>PAAELEARQFDPDSFKNKWLELHNNERT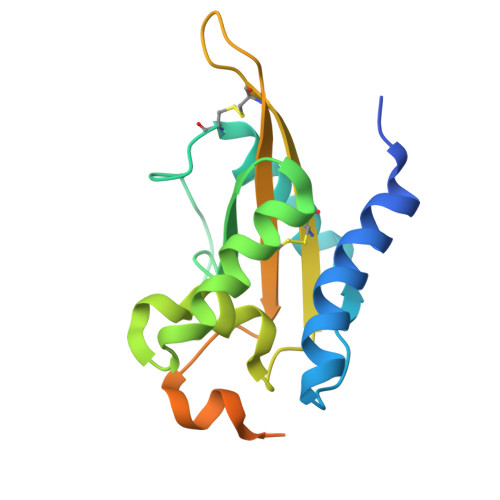TRQLDSLEWDGDLAWKAQQVATQCNVDNPQLWGDNGASFNIGRYTKEQAFAEWTATSGSFPDDRSIPWQRIVANSAQKVGCGEATCVLEGDMAYTVNVCYYDPPLSDYYTNAGDNVRVPSLALLNLDLTTPFCNLPVNGSNDLDIRE[7x]> PPHPQDLEITKLPNGLVIASLENYSPGSTIGVFIKAGSRYENSSNLGTSHLLRLASSLTTKGASSFKITRGIEAVGGKLSVESTRENMAYTVECLRDDVEILMEFLLNVTTAPEFRPWEVADLQPQLKIDKAVAFQNPQTHVIENLHAAAYRNALADSLYCPDYRIGKVTSVELHDFVQNHFTSARMALVGLGVSHPVLKNVAEQLLNIRGGLGLSGAKAKYRGGEIREQNGDSLVHAAIVAESAAIGGAEANAFSVLQHVLGANPHVKRGLNATSSLYQAVAKGVHNPFDVSAFNASYSDSGLFGFYTISQAAYAGQVIKAAYNQVKTIAQGNVSNENVQAAKNKLKAKYLMSVESSEGFLEEVGSQALAAGSYNPPSTVLQQIDAVADADVIKAAKKFVSRQKSMAASG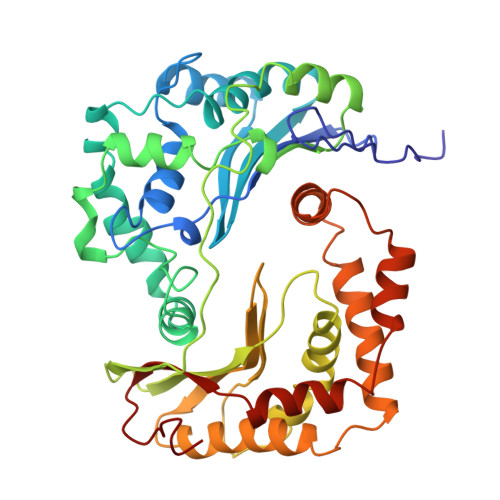NLGHTPFVDEL>MKDGMRVGERFTHDFVVPPHKTVRHLYPESPEFAEFPEVFASGFMVGLMEWACVRAMAPYLEPGEGSLGTAICVTHTAATPPGLTV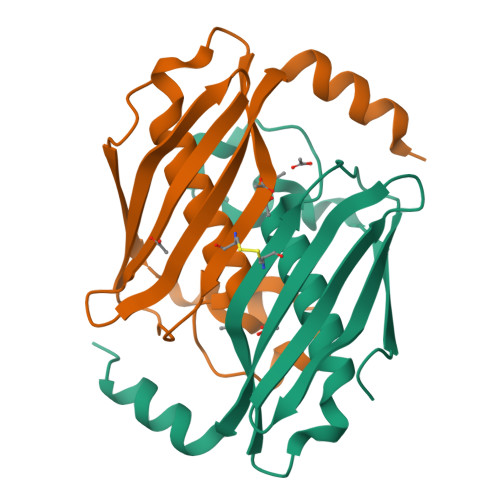TVTAELRSVEGRRLSWRVSAHDGVDEIGSGTHERAVIHLEKFNAKVRQKTPAG[2x]>KKAVINGEQIRSISDLHQTLKKELALAEYYGENLDALWDALTGWVEYPLVLEWRQFEQSKQLTENGAES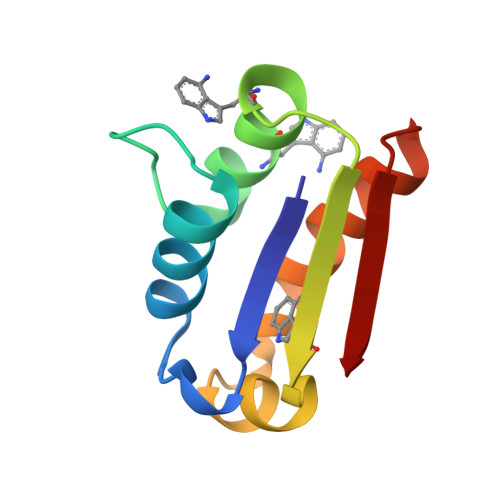VLQVFREAKAEGADITIILS[2x]> MDVASLPGKLADCSSKSPEECEIFLVEGDSAGGSTKSGRDSRTQAILPLRGKILNVEKARLDRI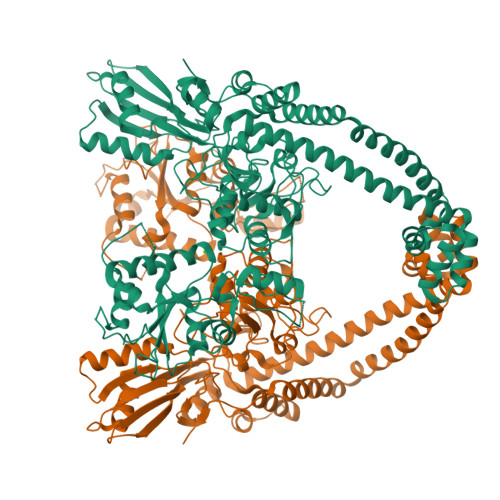LNNNEIRQMITAFGTGIGGDFDLAKARYHKIVIMTDADVDGAHIRTLLLTFFYRFMRPLIEAGYVYIAQPPLYKLTQGKQKYYVYNDRELDKLKSELNPTPKWSIARYKGLGEMNADQLWETTMNPEHRALLQVKLEDAIEADQTFEMLMGDVVENRRQFIEDNAVYANLDFAELPQSRINERNITSEMRESFLDYAMSVIVARALPDVRDGLKPVHRRILYGLNEQGMTPDKSYKKSARIVGDVMGKYHPHGDSSIYEAMVRMAQDFSYRYPLVDGQGNFGSMDGDGAAAMRYTEARMTKITLELLRDINKDTIDFIDNYDGNEREPSVLPARFPNLLANGASGIAVGMATNIPPHNLTELINGVLSLSKNPDISIAELMEDIEGPDFPTAGLILGKSGIRRAYETGRGSIQMRSRAVIEERGGGRQRIVVTEIPFQVNKARMIEKIAELVRDKKIDGITDLRDETSLRTGVRVVIDVRKDANASVILNNLYKQTPLQTSFGVNMIALVNGRPKLINLKEALVHYLEHQKTVVRRRTQYNLRKAKDRAHILEGLRIALDHIDEIISTIRESDTDKVAMESLQQRFKLSEKQAQAILDMRLRRLTGLERDKIEAEYNELLNYISELETILADEEVLLQLVRDELTEIRDRFGDDRRTEIQLG Human RNA exoribonuclease 2 (Rexo2) is an evolutionarily conserved 3′-to-5′ DEDDh-family exonuclease located primarily in mitochondria. Rexo2 degrades small RNA oligonucleotides of <5 nucleotides (nanoRNA) in a way similar to Escherichia coli Oligoribonuclease (ORN), suggesting that it plays a role in RNA turnover in mitochondria. Rexo2 forms a homodimer and interacts mainly with the last two 3′-end nucleobases of substrates by hydrophobic and π−π stacking interactions via Leu53, Trp96, and Tyr164, signifying its preference in binding and degrading short oligonucleotides without sequence specificity. Rexo2 contains four strictly conserved DEDD residues (D47, E49, D147, D199) for binding two metal ions, as well as a general base (H194) in the active site for hydrolysis of the phosphodiester bonds in nucleic acid substrates.

We obtained three complex cocrystals, referred to as Rexo2–RNA (Rexo2–D199A bound with a 12-nt U12 RNA and Mg2+), Rexo2–DNA1 (wild-type Rexo2 bound with a 5-nt T5 DNA), and Rexo2-DNA2 (Rexo2–D199A bound with a 10-nt T10 DNA and Mg2+). Similarly, in Rexo2–DNA1 and Rexo2–DNA2 complex structures, DNA substrates were bound only in the active site of protomer B but not observed in protomer A. In contrast, 7 nt (T4–T10) were observed in Rexo2–DNA2 complex, with additional interactions of the phosphate backbone (P5) with side chains of Lys189 and Lys190, and π–π stacking interactions between T4 nucleobase and Phe186. Due to crystal packing, we also noted the π–π stacking interactions between T5 nucleobase and Tyr122 of the neighboring Rexo2 molecule. The electrostatic surface of Rexo2 reveals a basic surface extending from the active site within which lie the two lysine residues (Lys189 and Lys190), suggesting that Rexo2 also binds long oligonucleotides for degradation. However, based on comparison of the three complex structures, Rexo2 appears to interact primarily with the last two 3′-end nucleotides, providing the structural basis for its preference for binding and degrading small oligonucleotides. The crystal structures of Rexo2 in complex with DNA reveal a similar DNA oligonucleotide-binding mode to that for RNA.

>AASMAQRMVWVDLEMTGLDIEKDQIIEMACLITDSDLNILAEGPNLIIKQPDELLDSMSDWCKEHHGKSGLTKAVKESTITLQQAEYEFLSFVRQQTPPGLCPLAGNSVHEDKKFLDKYMPQFMKHLHYRIIDVSTVKELCRRWYPEEYEFAPKKAASHRALDAISESIKELQFYRNNIFK[2x]> MAGEGEDEQQEQGKGSHLVLLPLPFQGHINPMLQLANLLHSKGFSITIIHPQLNSPNPSDYPNLNFEIIPDGFSEPQRTGIKIIELLSAVNTNCEAP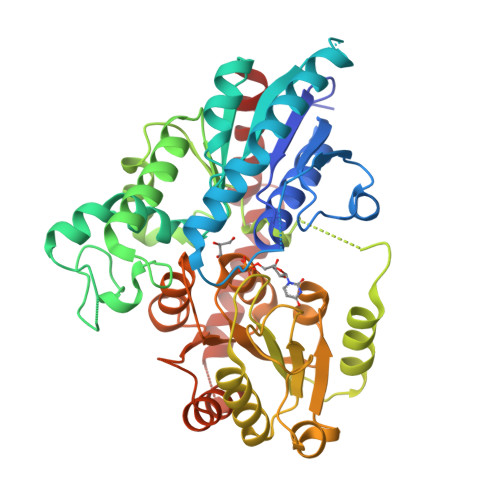LRECLARLQAANPLNPISCLITDAILYSTQTIAEDLGLPRIVLRTSSPFSFLAFAMYSHLKAKGYLPIQDHRSEISVVELPPLRVKDLPGYPNTDVNAHSQFFEKIVNTTRSATAVILNSSDHLERAILPELHREFPIPIFFVGPLCKSSSSVSSNRLSENEQSCLDWLDKQESRSVLYVSFGSVTEMEEADLAETAWGLANSEQPFLWVIRPGLVTGSERTWPHLPEGFAEKTKGKGWVVKWAPQQKVLVHPAVGGFWTHAGWNSTLEGICSGVPMICWPRNGDQTVNARLVSCSWKVGLQLEGDRLERGEIEKGLRKLMADKEGEEMRERARVLKETAELCVIKGGSSYVAMNKLVNHILSL>MQLTRLVQVDCPLGPDVL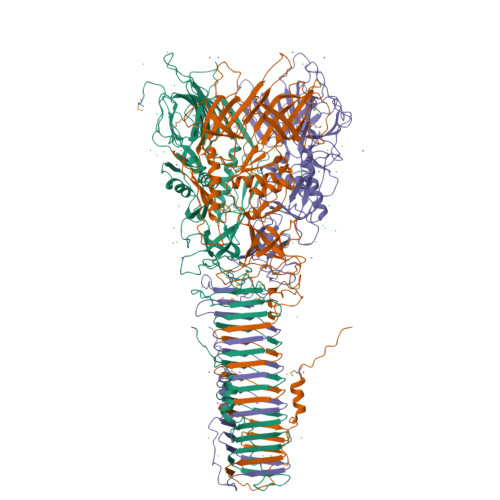LLQRMEGREELGRLFAYELHLVSENPNLPLEQLLGKPMSLSLELPGGSRRFFHGIVARCSQVAGHGQFAGYQATLRPWPWLLTRTSDCRIFQNQSVPEIIKQVFRNLGFSDFEDALTRPYREWEYCVQYRETSFDFISRLMEQEGIYYWFRHEQKRHILVLSDAYGAHRSPGGYASVPYYPPTLGHRERDHFFDWQMAREVQPGSLTLNDYDFQRPGARLEVRSNIARPHAAADYPLYDYPGEYVQSQDGEQYARNRIEAIQAQHERVRLRGVVRGIGAGHLFRLSGYPRDDQNREYLVVGAEYRVVQELYETGSGGAGSQFESELDCIDASQSFRLLPQTPVPVVRGPQTAVVVGPKGEEIWTDQYGRVKVHFHWDRHDQSNENSSCWIRVSQAWAGKNWGSMQIPRIGQEVIVSFLEGDPDRPIITGRVYNAEQTVPYELPANATQSGMKSRSSKGGTPANFNEIRMEDKKGAEQLYIHAERNQDNLVENDASLSVGHDRNKSIGHDELARIGNNRTRAVKLNDTLLVGGAKSDSVTGTYLIEAGAQIRLVCGKSVVEFNADGTINISGSAFNLYASGNGNIDTGGRLDLNSGGASEVDAKGKGVQGTIDGQVQAMFPPPAKGLEHHHHHH[2x]2-methylbenzene-1,4-diol | C7 H8 O2 | 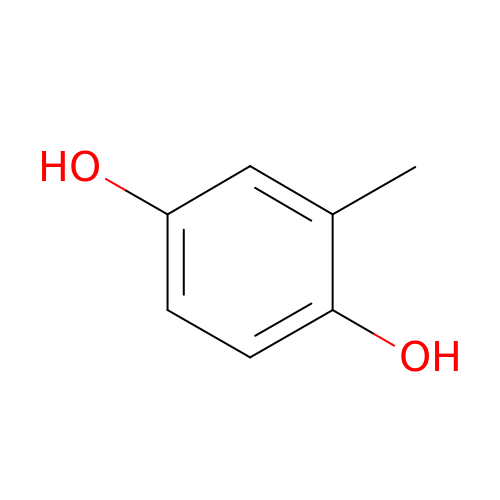CNHDIAIOKMXOLK-UHFFFAOYSA-N>MTSSGETIVEVDLSKEDDAFLAGHTIDGRILFPATGYMTLAWQTFAKMQGSEFHKTPVVMENLVFHRATILNKNAVVKFGINFFDGTGAFEICESGSLAVSGKITIPESIDNEELPLEEQTPSAVAKELGTNDVYKELRLRGYDYGGIFRGIVRSDTVASTGKLQWVDNWISFMDTMLQFSILSKNLRELYLPTRIERAVINPAKHFELLSALTKEEQVETGLPVQWYSDINVIKSAGVELRGLKANLAQRRPGTQAPPTLERYQFVPNINTTDLNENSEKARLHALDVAIQVIIENSSGAVKLKGVELANGRNPDVLVANRLLQIIEGEPVLTGDVAVVTSNNNEETITAALGDSGVRVVSKDVLKEPVEQNCHFVFGIDVLSRPDTKTLENSIASIRENGFLILEETLPTYTKTGRALLTKFGFVAVQEQSLGATRVLVLARKAVDLKTRKSVVVVATEQNFNWVDDLKAALATAATEEQYVYVVCQGEELFGAVGLMTCIKNENGGKLARLVFVQDAKAEKFSLTSTLYRQQLEKDLISNVLKNGAWGTFRHLKLETQQATLQVEHAYVNALVKGDLASLKWIEAAQAD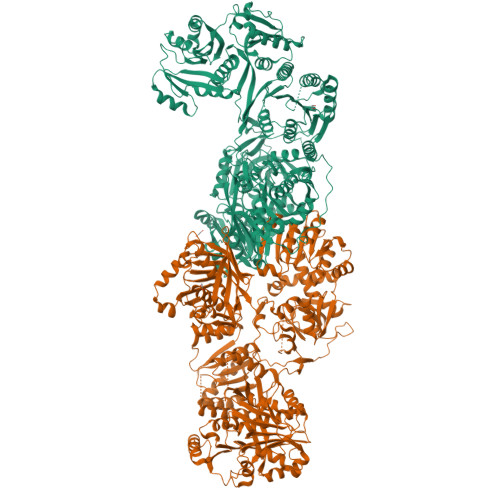TAATVDKNLETCTVYYAPINFRDVMLTSGKLAADALPGDLAEQDCVLGLEFAGRDTQGRRVMAMVPAKSLATTCVASKRMMWQIPEKWTMEEASTVPCVYSTVYYALVVRGQMKKGEKILIHAGSGGVGQAAISVALAHGLTVFTTVGSKEKREFLLKRFPKLQERNIGNSRDTSFEQLVLRETKGRGVDLVLNSLSEEKLQASIRCLGLNGRFLEIGKFDLSNNSPLGMSVFLKNTSFHGILLDSVMEGEEEMQNQVVSLVAEGIKTGAVVPLPTSVFNDQQVEQAFRFMASGKHIGKVVIKVRDEEAGKKALQPKPRLINAIPRTYMHPEKSYILVGGLGGFGLELTNWLVTRGARYIVLTSRSGVKTGYQGLMIRRWQERGVKVVIDTSDVTTAAGAKKLLENSNKLALVGGIFNLAAVLRDALIEDQTAKDFKTVADPKVTATKYLDQFSRDICTELDYFICFSSVSCGRGNIGQTNYGLANSAMERICEQRQVSGFPGTAIQWGAIGDTGLVLENLGDNDTVIGGTLPQRMPSCLQTIDLFLQQPHPVVASMLEVLFQGPHPAFLYKVVSHHHHHHHHHH[2x]> GGKKKNYQRYPKPPYSYLAMIAMVIQNSPEKKLTLSEILKEISTLFPFFKGNYKGWRDSVRHNLSSYDCFVKVLKDPGKPQGKGNFWTVEVNRIPLELLKRQNTAVSRQDETIFAQDLAPYIFQG

Forkhead box H1 (FoxH1) is an essential maternal pioneer factor during embryonic development that binds to specific GG/GT-containing DNA target sequences. The members of the FOX transcription factor family share the presence of the forkhead domain (FH), which interacts with DNA (InterPro entry IPR001766). Most FOX proteins recognize the canonical forkhead DNA motif TRTTTRY (R = A/G, Y = C/T). In contrast, FoxH1 recognizes the TGTG(G/T)ATT sequences in several cis-regulatory elements, such as in Gsc, Eomes, Nodal, Mixl, and FoxA2, to confer activin regulation in vivo.

To decipher how FoxH1 selects GK sites and how the extended domain contributes to DNA binding, we determined the crystal structures of FoxH1 proteins from three selected species, H. sapiens, D. rerio, and X. laevis, bound to a 16 bp native sequence belonging to the mouse Gsc promoter containing the GG site. The three GG complexes were refined at 0.98 Å (D. rerio, C2 space group), 1.47 Å (H. sapiens, P21 space group), and 2.8 Å resolution (X. laevis, P212121 space group). The atomic resolution data of the two GK structures, with average B-factors of 19.3 and 17.0 Å2, respectively, allowed us to determine the position of each atom of the 32 DNA nucleotides, 120 protein residues, and 360/219 water molecules in the GG/GT structures, respectively. In the FoxH1 complexes bound to the GG site, Wing1 and Wing2 are well-ordered and, together with the N-terminal loop, they contribute to specific recognition of DNA. Wing2 starts with two 310 helices (H4 and H5), followed by an isolated β-bridge formed by Lys185 and Asp202 in zebrafish and by Arg121 and Asp143 in humans. The Wing2 region also interacts with minor groove 1, directly with the backbone (Gln187 to A6′, Asn188 to A16, and Arg193 to G15) and indirectly by guiding the N-terminal loop also towards this groove, where it establishes several base-specific HBs, for instance, between Tyr92 and A6′, and between Arg94 and T12 and G13. These interactions are well-defined, as depicted in the snapshot showing the atomic-resolution 2Fo-Fc electron density maps of the zebrafish GG complex contoured at 1.0 sigma.>[2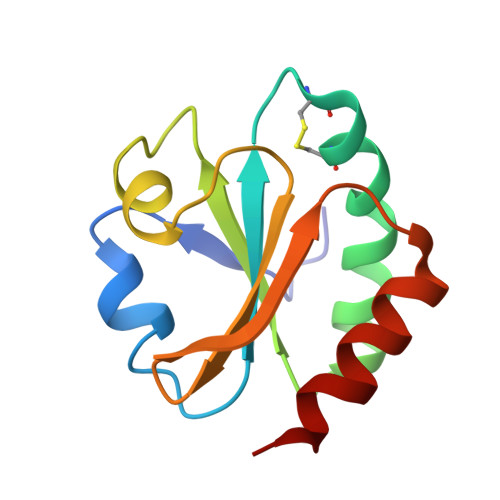x]GSDKIIHLTDDSFDTDVLKADGAILVDFWAEWCGPCKMIAPILDEIADEYQGKLTVAKLNIDQNPGTAPKYGIRGTPTLLLFKNGEVAATKVGALSKGQLKEFLDANLAAA>HHHHHHDITFRNIRFRYKPDSPVILDNINLSIKQGEVIGIVGRSGSGKSTLTKLIQRFYIPENGQVLIDGHDLALADPNWLRRQVGVVLQDNVLLNRSIIDNISLANPGMSVEKVIYAAKLAGAHDFIS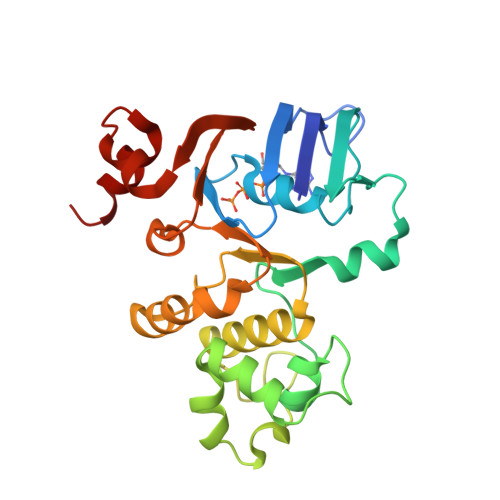ELREGYNTIVGEQGAGLSGGQRQRIAIARALVNNPKILIFDQATSALDYESEHVIMRNMHKICKGRTVIIIAHRLSTVKNADRIIVMEKGKIVEQGKHKELLSEPESLYSYLYQLQSD[4x]>[4x]GSMLTIGQLARIFEISTKTLRHYDAIGLFVPARTGSDNGYRYYQPEQIEQLSRILALRRLDVPLEAIDRLKRDGALDDPQRLRHFLQRHQHTLREEISARQRLLAELDR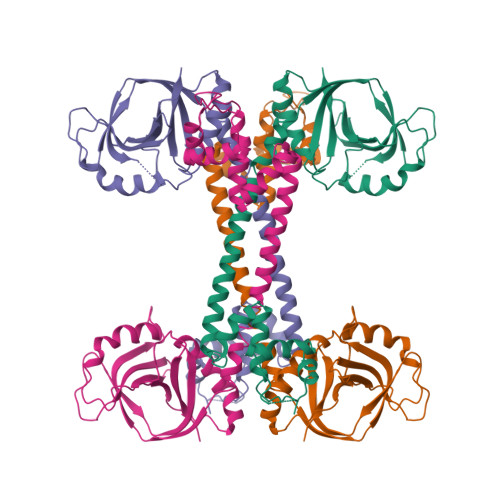TLATLAHWRIRNMHARIVERPAFSVVGMEYFGSAPGDTIGQLWERFIPREHEIAGKHDPEVSYGICAQQPNGEFHYVAGFEVQEGWPVPEGMVRFQVPAQKYAVFTHKGTAPQIAESFQAIYSHLLAERGLEPKAGVDFEYYDQRFRGPLDPNSQVDLYIPIY> PVMHPHGVPPSHRPWQMKDLQAIKQEVSQAAPGSPQFMQTIRLAVQQFDPTAKDLQDLLQYLCSSLVASLHHQQLDSLISEAETRGITGYNPLAGPLRVQANNPQQQGLRRE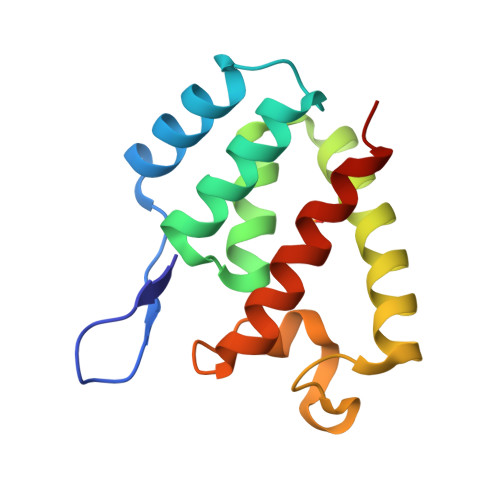YQQLWLTAFAALPGS>MAPQEQASSSQQDDAPPKTPNVVEPYKGEVAICGLSGRYPESANVGELEYNLFNKIDMVTIDNRRWEPGYLGTPERMGKVKTITDFDAEFFGVHTKGAQTMDPMLRNLLEVVYEAIVDAGESLESMKGTRTGVYIGVSNNEVDTAYMKNWTDDDAYMVQGCHHSMYPNWISFFFDFSGPSTAYNTACSTSLVCLDAAERHLRMGVIDNAIVGGSNFIYRPATTKLFMGMNFLGSSTCKAFDESGDGFVRGEVASAILLKKADTAKRVYCTLVGSMLNNDGNQTNGILYPNSEAQEQLMTDIYSTHKIDANEVKYFECHGTG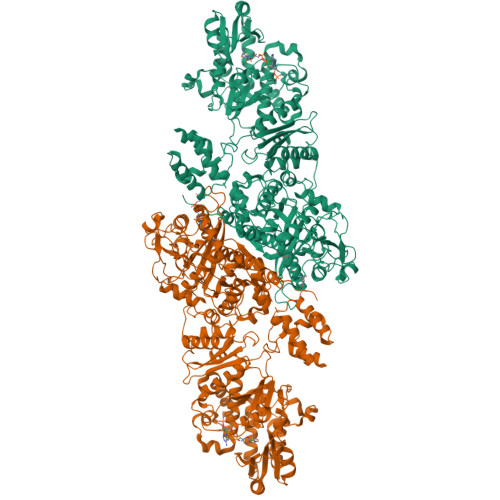TQAGDPNETRAICNAVCKGKKDPLLIGSIKSNLGHGETASGINGISKVIITMHSRQIPPNLHFKNPNPKIPGLFDGRLKVVTETTPFDGGLIAINSFGMGGTNAHAIFRSFDKRAEPHPASDKPRLFTYCARTEEGLQKIFEEAHKHASNVEFHALCQESANTKPKSLPYRGATILNAEGEYTEIQKCPSKAREVWFVYSGMGSQWVGMGRSLMALDVFRQSIEETAAILSPFGVDLMSLLMDGTEDKLKEIMPPFICINAIQLALTDLLNSMGIVPDGLVGHSLGEVGCAYADGCLTRREAILSAFWRAKAVIDCEVKPGKMAAVELTWEEAKRLCPPGVVAACHNSQDSVTISGGAQEMTKFMAELSAQGVTVKEVNSNNISYHSSFMTEPAAYLKKGLEKEIVPKPRSKKWISTSIPEERWGNPEAQTADASYQANNLLSSVLFYEGLQKIPSNAIAIEIAPAGLLQSVIKKSLGQDCTIVALQKRKSPNNLEVFFSALGKCYSHGVPMNPLGLYPAVQFPVSIDTPMLSSMVSEAWDHSAKWRVPLVEEFEYGSGSSSDNVIDIDLSEDSPENYLLEHAVDGRMLFPATGTLVLAWKTLAKLKGVEFEQLGVQMTNVQIHQALFLNPGGKTTVSVSVMPITGEFQVRDGESLISSGVITSSEGRLLETDQHMKKGSVLDGKPDKELLFTKEIYREFLLRGYEYGAAFQGIQRASLDATDTDIRWDGRWISYLDTVLQMYLLSKPGTHQALPTLLESVTIDPRVHPAQPPEGTTEFQVLPGKWDPVLQIAAAGGVEIRSCHSIRASRRLNHDPPILEDFAFAPYVDPRPSDRSAAAVTPALRDYADACFEFSRQGMKRWLENDKNNVLPNKEEIKEALAMANKHASTPQAASNFASAKATLEALVNNKNGHRLPNHGLFEMLDIAFSEPLEGDYWDRLRMKLHDVRTYLWDDPIIAALESPDIVKLVMETVSDNVNQQVMEILEVGAARGPYYRQAIPKALEYFSIKDWQYTVADQGFVEDAAEFPVKMMQFDPLDPANFPAELTESCDLLVLKWNLQMQVDLDAAITEFSKMIKPGGFLLVLENGTRLSTFFPIKAIVSASLGGKGGPEGDRAMGCFYTDAQWSALFARHGFEQIMHIPDGIAVSMFLLRKPFEPSVAPIIINVDDLECSWLEEVQARCAELQDSHKDSRLWLVANTELSGVLGFLRSLVWEFGSEKLRCIQIDDATAGPNPPKISADSADFKELVRKDLAYNVFKNGKWGTYRGFVISDADRQKERPSEYVYADWLSAGDMSSLRWFDSPLKTGHNNGMLGSKMAHKLETETCSVYYAGLNLRDIILANGTIQRDILPEETFFKEGVLGVEFSGRNSSGKRVMGLCPPPALATTVKCPVSSLWSVPDQWTLEEAATVPLAYATAYYCLVSEGGVQKGATVFIHAGASVVGQASIAVALSYNCEIFTLTKNSDETALLKSMYPQLNDRNFCSSEDCSFEKYIRKETKGSGVDVVINTLRGKFLKASRRLLSKKGKFVDIGFKVDSNTQIAYYTREHPDLRFQLDALLESQGPEWTRLFDLVQAGIHSGVVKPLKRAVYSMDKIVDAFKTVEAEREAGKIVIKIRDEERQKVCPTPRTSFPAIHRTCFHPDKSHILVGGMGGMGLETAHWMVLRGAKKLILTSRYGITTGYQARKIAFFKQLGVEVEVLALSVNTRKAADKVFEHALKMGPVGGIFNMAMVLYNDDFLKMNREQFLKPLESKITMTMLLDDKSREKPVRDTLDHFVMFSSLIVSGGHLGQANYAFGSTVLEKICERRKRDGLPVTTPQWASIADVGTVALMGTGNETIICRKYPQRFFNVLSVFDFMMSSDNVVTISYVLVEKSMGVAAGEESMVDQVLRAVGKVLGIKDVSSVDGDKEFIDMGVDXLMSVEIKQALERDAGLVISTKDTQLMTFNTLRSMVKGSHVHHHHHH[2x]>[8x]MTRTLPPGVSDERFDAALQRFRDVVGDKWVLSTADELEAFRDPYPVGAAEANLPSAVVSPESTEQVQDIVRIANEYGIPLHPVSTGKNNGYGGAAPRLSGSVIVKTGERMNRILEVNEKYGYALLEPGVTYFDLYEYLQSHDSGLMLDCPDLGWGSVVGNTLDRGVGYTPYGDHFMWQTGLEVVLPQGEVMRTGMGALPGSDAWQLFPYGFGPFPDGMFTQSNLGIVTKMGIALMQRPPASQSFLITFDKEEDLEQIVDIMLPLRINMAPLQNVPVLRNIFMDAAAVSKRTEWF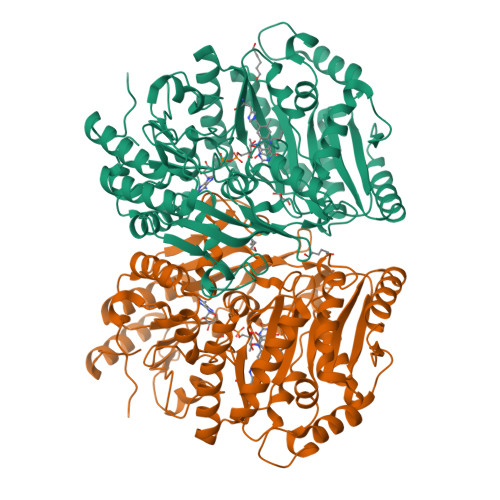DGDGPMPAEAIERMKKDLDLGFWNFYGTLYGPPPLIEMYYGMIKEAFGKIPGARFFTHEERDDRGGHVLQDRHKINNGIPSLDELQLLDWVPNGGHIGFVPVSAPDGREAMKQFEMVRNRANEYNKDYMAQFIIGLREMYHVCLFIYDTADPEAREEILQMTKVLVREAAEAGYGEYRTHNALMDDVMATFNWGDGALLKFHEKIKDALDPNGIIAPGKSGIWPQRFRGQNL>[8x]SLRLIATEEAVTFQPVVDALRAHSRTDDASLDMILVRDVYGDEPARPAM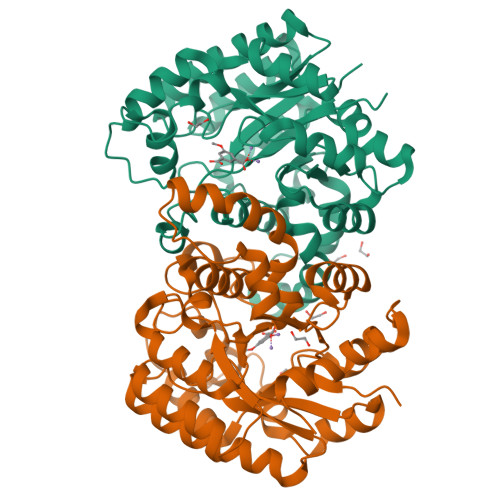IGRLSDVTGERLAEMDSNGVDMHLLSLTAPGVQMFDAETGTRLARIANDLMAQTVAANPTRFAGLGTFAPQDPASAAREIERVATQLRLNGLVINSHTNDLYYDDPFFHPVFEAIEASGLALYIHPRAPSKQIDRAFRDYGMNSAIWGYGIETSTNAVRMILSGLFDRFPRLKIVLGHMGEAIPFWLWRLDYMHGNATTFGGAPKLKLKPSEYFRRNFAITTSGVESHAALRYSIEVLGPENVMWAIDYPYQPMAPAVQFIRTAPIPEDVKAMVAGGNAARIFRIT> ISPIFQGGSYQLNNKSIDISSLLLDKLSGESQTVVMKFKADKPNSLQALFGLSNSKAGFKNNYFSIFMRDSGEIGVEIRDAQKGINYLFSRPASLWGKHKGQAVENTLVFVSDSKDKTYTMYVNGIEVFSETVDTFLPISNINGIDKATLGAVNREGKEHYLAKGSIDEISLFNKAISDQEVSTIPLSNPFQLIFQSGDSTQANYFRIPTLYTLSSGRVLSSIDARYGGTHDSKSKINIATSYSDDNGKTWSEPIFAMKFNDYEEQLVYWPRDNKLKNSQISGSASFIDSSIVEDKKSGKTILLADVMPAGIGNNNANKADSGFKEINGHYYLKLKKNGDNDFRYTVRENGVVYNETTNKPTNYTINDKYEVLEGGKSLTVEQYSVDFDSGSLRERHNGKQVPMNVFYKDSLFKVTPTNYIAMTTSQNRGESWEQFKLLPPFLGEKHNGTYLCPGQGLALKSSNRLIFATYTSGELTYLISDDSGQTWKKSSASIPFKNATAEAQMVELRDGVIRTFFRTTTGKIAYMTSRDSGETWSKVSYIDGIQQTSYGTQVSAIKYSQLIDGKEAVILSTPNSRSGRKGGQLVVGLVNKEDDSIDWKYHYGIDLPSY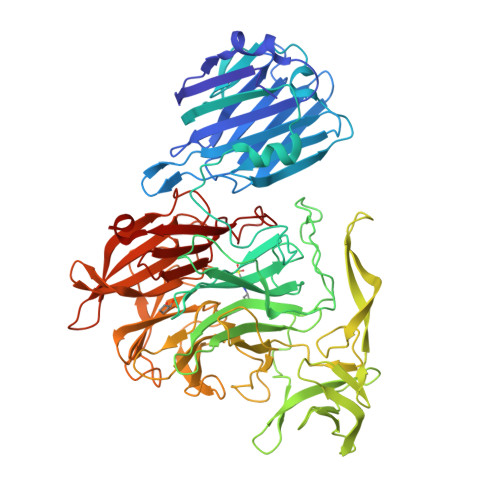GYAYSAITELPNHHIGVLFEKYDSWSRNELHLSNVVQYIDLEINDLT> GLENSGNARDGPLDFEESYKGYGEHELEENDYLNDETFGDNVQVGTDFDF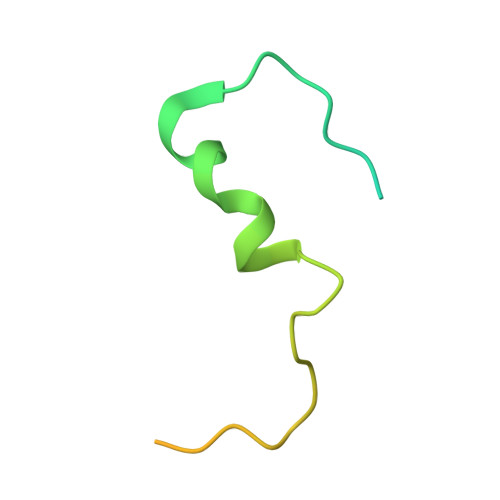GNPHSSGSSGNAIGGNGVGATARSY> GPLSVAASHCQ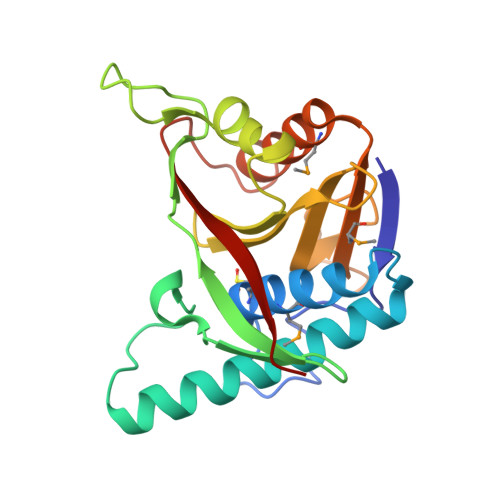SDVRYDSNSRNRQCTCNALMFLAVHNESNQLQSADLDCVLQKGDAVYSSVKRSLQNKGQFVHDFLNFDELPSTIETNSRCYNIVKHPQRFGFLKDTPALGEYQNLENTLQCLKSGLTDALLLCGGSCIAVFRDRTGRFGYFDSHSRTPDGKYTGEKSGTAVMLTFLHLKAMVEKLLQLFQGCLQLSDQEQFDLLPVSFIEIT>MPACCSWNDVFQYETNKVTRIQSVNYGT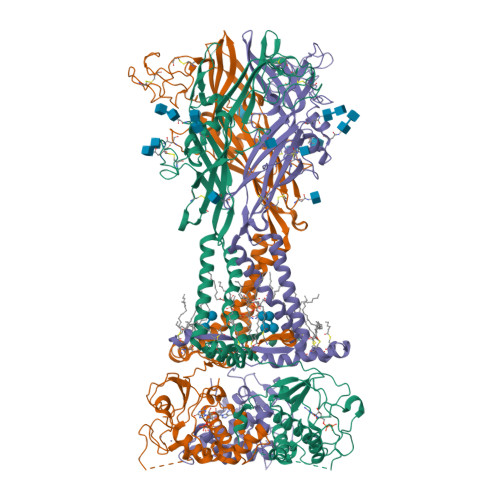IKWILHMTVFSYVSFALMSDKLYQRKEPLISSVHTKVKGVAEVTENVTEGGVTKLVHGIFDTADYTLPLQGNSFFVMTNYLKSEGQEQKLCPEYPSRGKQCHSDQGCIKGWMDPQSKGIQTGRCIPYDQKRKTCEIFAWCPAEEGKEAPRPALLRSAENFTVLIKNNIDFPGHNYTTRNILPGMNISCTFHKTWNPQCPIFRLGDIFQEIGENFTEVAVQGGIMGIEIYWDCNLDSWSHRCQPKYSFRRLDDKYTNESLFPGYNFRYAKYYKENGMEKRTLIKAFGVRFDILVFGTGGKFDIIQLVVYIGSTLSYFGLATVCIDLIINTYASTCCRSRVYPSCKCCEPCAVNEYYYRKKCEPIVEPKPTLKYVSFVDEPHIWMVDQQLLGKSLQDVKGQEVPRPQTDFLELSRLSLSLHHSPPIPGQPEEMQLLQIEAVPRSRDSPDWCQCGNCLPSQLPENRRALEELCCRRKPGQCITTSELFSKIVLSREALQLLLLYQEPLLALEGEAINSKLRHCAYRSYATWRFVSQDMADFAILPSCCRWKIRKEFPKTQGQYSGFKYPYSNSAVDAGLEVLFQ[3x]>[2x]MITQEMKDLINNQLAMVATVDAKGQPNIGPKRSMRL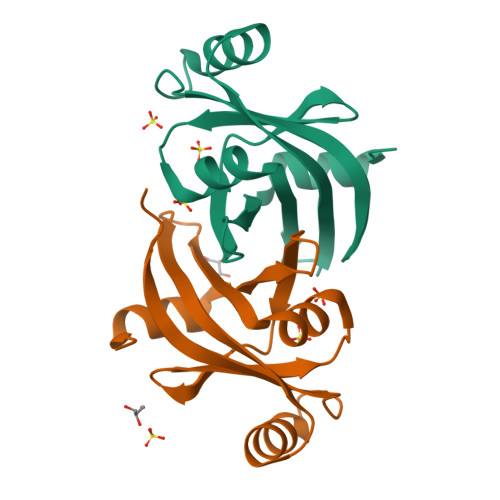WDDKTFIYNENTDGQTRINIEDNGKIEIAFVDRERLLGYRFVGTAEIQTEGAYYEAAKKWAQGRMGVPKAVGIIAVERIFNLQSGANAGKEINSESNKGELNSKLEGKPIPNPLLGLDSTRTGHHHHHH>[2x]MKIIALRSSLKLAARIAEELKTEPVMPDERRFPDGELYLRYDEDLTGHNIFIIGNTHSDAEVMEMILTLSAIQD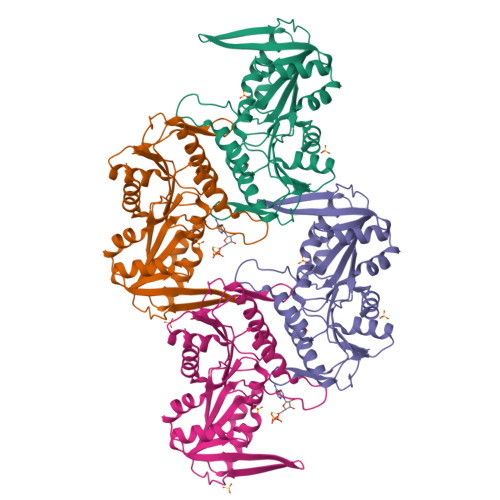YRTKSVNIIAPYYGYARQHQRYKNGEPISSQILTEIYSSYSNSIATVDIHDEKTLSYSKVKFSDLHANDAIVRYYKNVDVDYVVSPDDGGLARVADISAKLGKKHFFIEKKRIDDRTVEMKVPNVDVNGKKLLIVDDIISTGGTIAKSSGLLREKGASKIYVSAVHGLFVNGSENKILQNADEIHVTDTVESKFSDISVYQEVCNYIRDIDA>[2x]MSGAPPPSSGFAPRSYGQQPLSHAPRSSMMSVEYDGIPLPPPSIRSCGSQQYVTSYIPTGAAFPPSSVQDMISSMKSYASATDLVRTYSEIPSVEEALSTLDRAAAALNARRYRDALKLYLEGGYAMANVAERQANPKICNLLTSKGFETLNWCARLCDWIEGRIKEKHPRPGVHKVGIPVSNWDEDWVGPFMDEEEARRMWYTPVYCPHPIDFSNLGYRLRCVETGRRPRLMICITMYNEGPQQLKATLKKLANNLAYLKEQMPGDEKSLTGAFAGDDVWQNVLVCIVADGREQVHPKTLDYLEAIGLYDEDLLTINSAGIGAQCHLFEHTL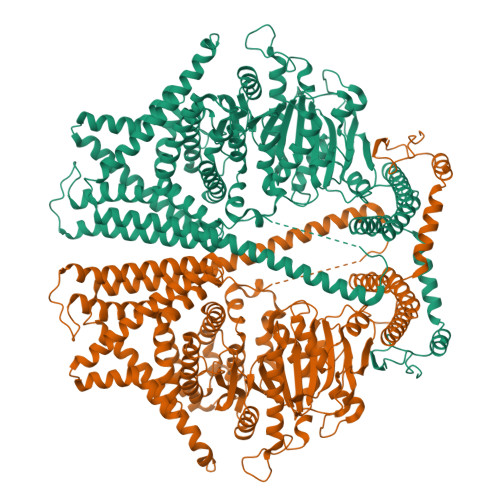QLSVNGKCLLPIQTVFALKENKASKLDSHHWYFNAFAEQIQPEYTAVMDVGTMLTKSALYHLLFAFERNHQIGGACGQLTVDNPFENLSNWVISAQHFEYKISNILDKSLESCFGFISVLPGAFSAYRYEAIRGAPLDAYFQTLNIELDVLGPFIGNMYLAEDRILSFEVVARKNCNWTMHYVKDAVARTDVPHDLVGLISQRKRWLNGAFFATLFSIWNWGRIYSESKHTFVRKMAFLVFYVYHLLYTAFGFFLPANLYLALFFIVFQGFQQNRLEFIDTSEYSQTVLDCAVYIYNFSYLFGLLMLIIIGLGNNPKHMKLTYYFVGAVFGLMMMLSSLVGAGIFFSTPATVHSIVVSILTVGVYFIASALHGEVHHIFMTFTHYTALIPSFVNIFTIYSFCNLQDLSWGTKGLHDDPLLAASLDETEKGDFKDVIAKRRALEELRREEKERVENRKKNFEAFRTNVLLTWAFSNLIFALFVVYFASSSTYMPVLYIFVASLNTCRLLGSIGHWVYIHTEGLRGRVIDKSECGNGTGRYPQNSYVQLEEHYAALAEDQRTYASGRTNASVRTVNDVSSAA>MSRSKRDNNFYSVEIGDSTFTVLKRYQNLKPIGSGAQGIVCAAYDA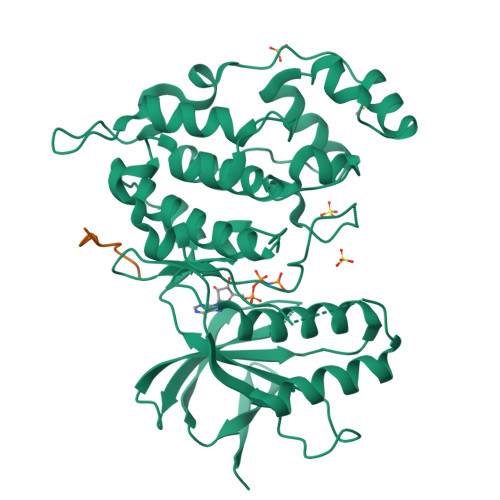ILERNVAIKKLSRPFQNQTHAKRAYRELVLMKCVNHKNIIGLLNVFTPQKSLEEFQDVYIVMELMDANLCQVIQMELDHERMSYLLYQMLCGIKHLHSAGIIHRDLKPSNIVVKSDCTLKILDFGLARTAGTSFMMTPYVVTRYYRAPEVILGMGYKENVDLWSVGCIMGEMVCHKILFPGRDYIDQWNKVIEQLGTPCPEFMKKLQPTVRTYVENRPKYAGYSFEKLFPDVLFPADSEHNKLKASQARDLLSKMLVIDASKRISVDEALQHPYINVWYDPSEAEAPPPKIPDKQLDEREHTIEEWKELIYKEVMDLE[4x];>[4x]QRPRPTLQLPLA>GAKPFGEKKFIEIKGRRMAYIDEGTGDPILFQHGNPTSSYLWRNIMPHCAGLGRLIACDLIGMGDSDKLDPSGPERYAYAEHRDYLDALWEALDLGDRVVLVVHDWGSALGFDWARRHRERVQGIAYMEAIAMPIEAADLPEQDRDLFQAFRSQAGEELVLQDNVFVEQVLPGWILRPLSEAEMAAYREPFLAAGEARRPTLSWPRQLPIAGTPADVVAIARDYAGWLSESPIPKLFINAEPGALTTGRMRDFCRTWPNQTEITVAGAHFIQE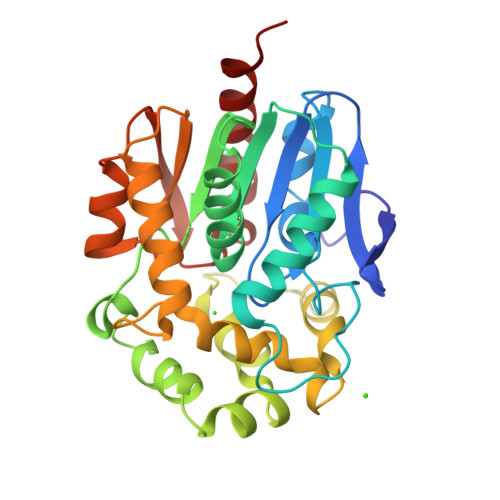DSPDEIGAAIAAFVRRLRPA[2x]> MKCPVCHQGEMVSGIKDIPYTFR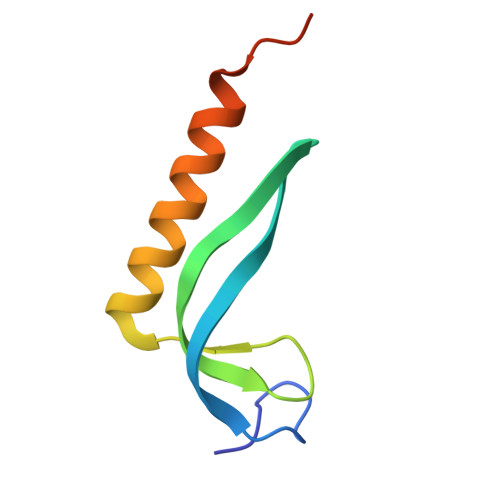GRKTVLKGIHGLYCVHCEESIMNKEESDAFMAQVKAFRASVNAETVAPEFIVK>[2x]QEHEPIGAQDERLSTLIHQRMQEAKVPALSVSVTIKGVRQRFVYGVADVASQKANTLDTVYELGSMSKAFTGLVVQILIQEGRLRQGDDIITYLPEMRLNYQGKPASLTVADFLYHTSGLPFSTLARLEN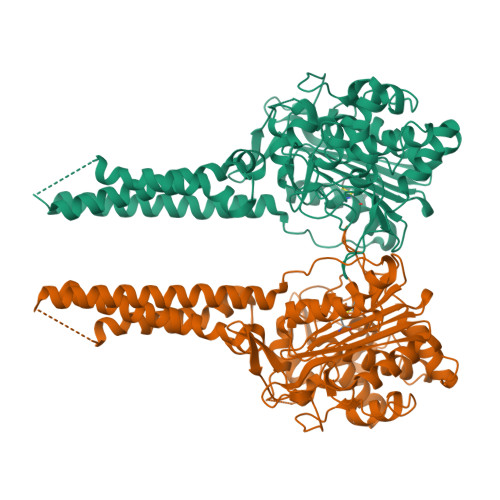PMPGSAVAQQLRNENLLFAPGAKFSYASANYDVLGAVIENVTGKTFTEVIAERLTQPLGMSATVAVKGDEIIVNKASGYKLGFGKPVLFHAPLARNHVPAAYIHSTLPDMEIWIDAWLHRKALPATLREAMSNSWRGNSDVPLAADNRILYASGWFIDQNQGPYISHGGQNPNFSSCIALRPDQQIGIVALANMNSNLILQLCADIDNYLRIGKYADGAGDAITATDTLFVYLTLLLCFWGAVVVVRGAFRVYRATAHGPGKQQRLRLRVRDYIIALAVPGLVAAMLYVAPGILSPGLDWRFILVWGPSSVLAIPFGIILLAFVLTLNHQIKRILLHNKEWDDEHHHHHHHHHH>[3x]TT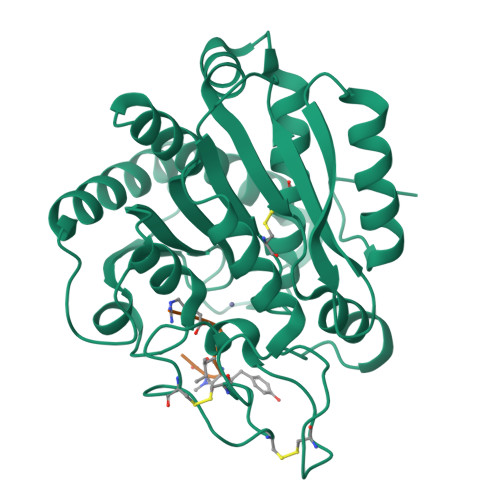GHSYEKYNNWETIEAWTKQVTSENPDLISRTAIGTTFLGNNIYLLKVGKPGPNKPAIFMDCGFHAREWISHAFCQWFVREAVLTYGYESHMTEFLNKLDFYVLPVLNIDGYIYTWTKNRMWRKTRSTNAGTTCIGTDPNRNFDAGWCTTGASTDPCDETYCGSAAESEKETKALADFIRNNLSSIKAYLTIHSYSQMILYPYSYDYKLPENNAELNNLAKAAVKELATLYGTKYTYGPGATTIYPAAGGSDDWAYDQGIKYSFTFELRDKGRYGFILPESQIQATCEETMLAIKYVTNYVLGHL;>RKIYAF[3x]HEPTYLFORMAMIDE 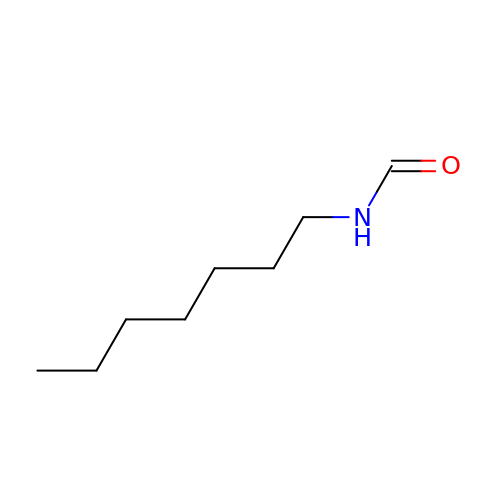| C8 H17 N O | YAUHDTOEJHVKJO-UHFFFAOYSA-N>[9x]MAQILPIRFQEHLQLQNLGINPANIGFSTLTMESDKFICIREKVGEQAQVVIIDMNDPSNPIRRPISADSAIMNPASKVIALKAGKTLQIFNIEMKSKMKAHTMTDDVTFWKWISLNTVALVTDNAVYHWSMEGESQPVKMFDRHSSLAGCQIINYRTDAKQKWLLLTGISAQQNRVVGAMQLYSVDRKVSQPIEGHAASFAQFKMEGNAEESTLFCFAVRGQAGGKLHIIEVGTPPTGNQPFPKKAVDVFFPPEAQNDFPVAMQISEKHDVVFLITKYGYIHLYDLETGTCIYMNRISGETIFVTAPHEATAGIIGVNRKGQVLSVCVEEENIIPYITNVLQNPDLALRMAVRNNLAGAEELFARKFNALFAQGNYSEAAKVAANAPKGILRTPDTIRRFQSVPAQPGQTSPLLQYFGILLDQGQLNKYESLELCRPVLQQGRKQLLEKWLKEDKLECSEELGDLVKSVDPTLALSVYLRANVPNKVIQCFAETGQVQKIVLYAKKVGYTPDWIFLLRNVMRISPDQGQQFAQMLVQDEEPLADITQIVDVFMEYNLIQQCTAFLLDALKNNRPSEGPLQTRLLEMNLMHAPQVADAILGNQMFTHYDRAHIAQLCEKAGLLQRALEHFTDLYDIKRAVVHTHLLNPEWLVNYFGSLSVEDSLECLRAMLSANIRQNLQICVQVASKYHEQLSTQSLIELFESFKSFEGLFYFLGSIVNFSQDPDVHFKYIQAACKTGQIKEVERICRESNCYDPERVKNFLKEAKLTDQLPLIIVCDRFDFVHDLVLYLYRNNLQKYIEIYVQKVNPSRLPVVIGGLLDVDCSEDVIKNLILVVRGQFSTDELVAEVEKRNRLKLLLPWLEARIHEGCEEPATHNALAKIYIDSNNNPERFLRENPYYDSRVVGKYCEKRDPHLACVAYERGQCDLELINVCNENSLFKSLSRYLVRRKDPELWGSVLLESNPYRRPLIDQVVQTALSETQDPEEVSVTVKAFMTADLPNELIELLEKIVLDNSVFSEHRNLQNLLILTAIKADRTRVMEYINRLDNYDAPDIANIAISNELFEEAFAIFRKFDVNTSAVQVLIEHIGNLDRAYEFAERCNEPAVWSQLAKAQLQKGMVKEAIDSYIKADDPSSYMEVVQAANTSGNWEELVKYLQMARKKARESYVETELIFALAKTNRLAELEEFINGPNNAHIQQVGDRCYDEKMYDAAKLLYNNVSNFGRLASTLVHLGEYQAAVDGARKANSTRTWKEVCFACVDGKEFRLAQMCGLHIVVHADELEELINYYQDRGYFEELITMLEAALGLERAHMGMFTELAILYSKFKPQKMREHLELFWSRVNIPKVLRAAEQAHLWAELVFLYDKYEEYDNAIITMMNHPTDAWKEGQFKDIITKVANVELYYRAIQFYLEFKPLLLNDLLMVLSPRLDHTRAVNYFSKVKQLPLVKPYLRSVQNHNNKSVNESLNNLFITEEDYQALRTSIDAYDNFDNISLAQRLEKHELIEFRRIAAYLFKGNNRWKQSVELCKKDSLYKDAMQYASESKDTELAEELLQWFLQEEKRECFGACLFTCYDLLRPDVVLETAWRHNIMDFAMPYFIQVMKEYLTKVDKLDASESLRKEEEQATETQPIVYGQPQLMLTAGPSVAVPPQAPFGYGYTAPAYGQPQPGFGYSM;>[6x]MADDFGFFSSSESGAPEAAEEDPAAAFLAQQESEIAGIENDEGFGAPAGSQGGLAQPGPASGASEDMGATVNGDVFQEANGPADGYAAIAQADRLTQEPESIRKWREEQRKRLQELDAASKVMEQEWREKAKKDLEEWNQRQSEQVEKNKINNRIADKAFYQQPDADIIGYVASEEAFVKESKEETPGTEWEKVAQLCDFNPKSSKQCKDVSRLRSVLMSLKQTPLSR

Clathrin-coated vesicles mediate trafficking of proteins and nutrients in the cell and between organelles. Proteins included in the clathrin-coated vesicles (CCVs) category include clathrin heavy chain (CHC), clathrin light chain (CLC), and a variety of adaptor protein complexes. Clathrin plays a major role in facilitating the formation of spherical vesicles by making closed fullerene-like cages of different sizes both in vitro and in vivo. Clathrin triskelia assemble into cages with pentagonal, hexagonal, and rarely heptagonal faces.

Here, using cryo-EM, we have determined the structures of natively assembled CCVs that include clathrin, adaptors, accessory proteins, and cargo. CCVs were purified from bovine brains in conditions that ensured that CHC cages do not disassemble during purification. The refined clathrin cages were further subjected to subparticle refinement to improve the resolution of the clathrin layer. Using subparticle reconstruction, we determined the structure of the most abundant vertex, which is asymmetric and formed from the intersection of two pentagonal faces and one hexagonal face. Atomic models were built of the mini-coat HPP asymmetric vertex. The model by Morris et al. that was built into their consensus C3 vertex [pentagonal-pentagonal-pentagonal (PPP)] was docked into our C1 vertex. In this rigid-body fit, the edge of the vertex that is between two pentagonal faces exhibits an accurate fit, while the two other edges with one hexagonal face do not enclose the model starting at positions close to the knee domain. This discrepancy is consistent with observations that the knee domain changes conformation to make hexagonal and pentagonal faces, while the proximal domain is stabilized by CLC. Consistent with their study, our structure also showed that the CLC C-terminal domain stabilizes the tripod domains that are critical for CHC trimerization.Recently, the ykkC RNA motif was identified as binding to multiple, chemically dissimilar ligands, which makes this specific scaffold a compelling target for structural studies of RNA evolvability (Sherlock et al., 2018a; 2018b; Nelson et al., 2017). Subtype 2b is responsive to phosphoribosyl pyrophosphate (PRPP), a precursor in purine biosynthesis. To address these questions of molecular recognition by RNA, we report the near-atomic resolution structure of a native ykkC 2b riboswitch in complex with PRPP via X-ray crystallography. We also convert this construct into a ppGpp aptamer with a single G96A mutation and present the structure of the mutant bound to ppGpp.

We mutated position 96 in the T. mathranii PRPP aptamer from guanosine to adenosine, generating the G96A mutant. Conversely, the G96A mutant binds ppGpp with an affinity equivalent to that of wild-type for PRPP (Kd = 1.8 ± 0.1 μM), but PRPP binding is abolished in the mutant up to 400 μM RNA (estimated Kd = 1600 ± 200 μM). The G96A mutation thus strikingly resulted in approximately a 40,000-fold switch in ligand specificity from PRPP to ppGpp. Having shown that the G96A mutant is a ppGpp aptamer, we solved its crystal structure in the presence of ppGpp to 3.1 Å resolution. Overall, the architecture of the G96A mutant is very similar to that of the wild-type aptamer. The positions of the 5′ and 3′ pyrophosphate groups of ppGpp are easily inferred from the available electron density data, which clearly show that the 5′ pyrophosphate occupies the former position of the pyrophosphate of PRPP. The guanine base of ppGpp is modeled in the syn conformation. In the syn conformation, the guanine base of the ligand forms three hydrogen bonds with C75 in a Watson-Crick base pair. Conversely, the S-turn motif is abolished in the G96A mutant, and no contacts are observed between A96 and other nucleotides. Rather, this region resembles a standard A-form helix with a single nucleotide bulge. The guanine of ppGpp replaces the flipped out guanosine of the former S-turn motif (G89/G96), revealing that the S-turn is a key center of functional plasticity in the ykkC RNAs.

>[4x]GUGAAAGUGUACCUAGGGUUCCAGCCUAUUUGUAGGUGUUCGGACCGAGCGGUACAGGUAUAUUUUUAUAUACCACACCUUAGGGACAAAAGCCCGAGAGGAUAGGUUUCACUCGUA> MARIPMASAGTSCVPGWAIPHNPLPSCRWYVTSRTCGIGPRLPWPE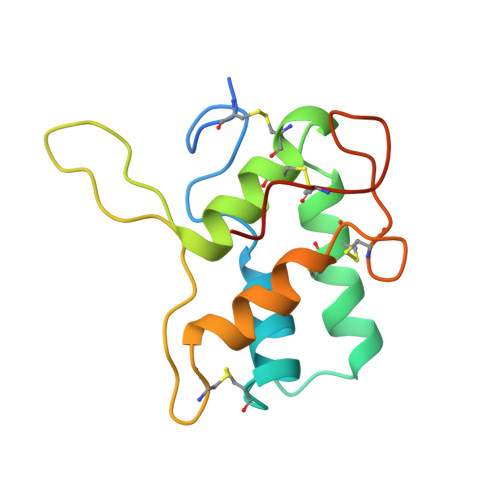LKRRCCRELADIPAYCRCTALSILMDGAIPPGPDAQLEGRLEDLPGCPREVQRGFAATLVTEAECNLATISGVAECPWILGGGTMPSK> MNILIFGPNGSGKGTQGNLVKDKYSLAHIESGGIFREH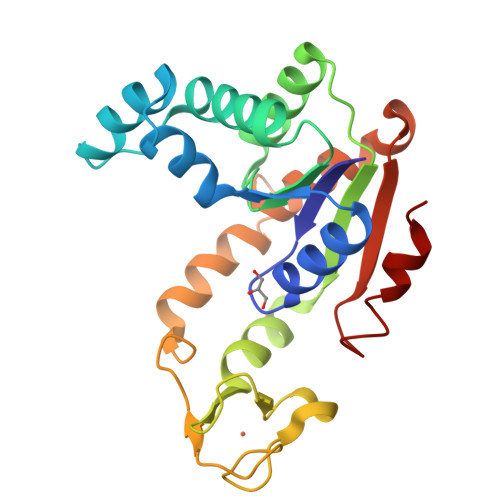IGGGTELGKKAKEFIDRGDLVPDDITIPMVLETLESKGKDGWLLDGFPRNTVQAQKLFEALQEKGMKINFVIEILLPREVAKNRIMGRRICKNNPNHPNNIFIEAIKPNGDVCRVCGGALSARADDQDEGAINKRHDIYYNTVDGTLAAAYYYKNMAAKEGFVYIELDGEGSIDSIKDTLLAQLA> MSLELGQAMVTVAGIGCRKGAASDAIIAAVRAAERAFGVTVDYLATAPLKADEAGLAEAAKGLSLSLEIVAQERLEAVAAETMTFSQASLDHSGSPSVSEAAALAAAGAGARLVA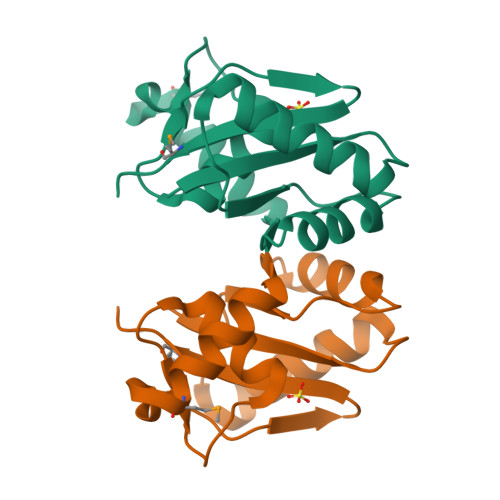PRLVVGDVTVAIAMTSDAPHGSRSAIEYGEQEEGHHHHHH N-(5-{4-[(1,1-dioxidothiomorpholin-4-yl)methyl]phenyl}[1,2,4]triazolo[1,5-a]pyridin-2-yl)cyclopropanecarboxamide | C21 H23 N5 O3 S | 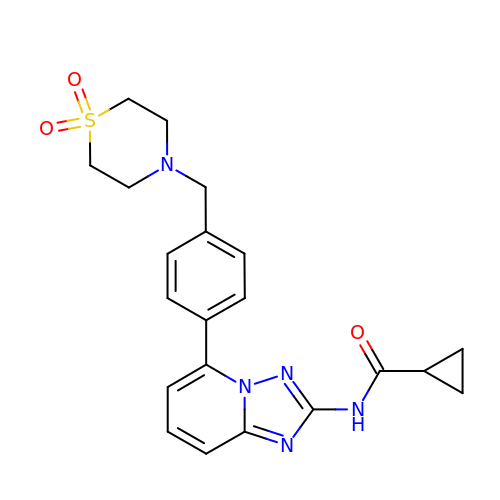RIJLVEAXPNLDTC-UHFFFAOYSA-N9-[(1R,6R,8R,9S,10R,15S,17R,18S)-3,9,12,18-tetrakis(oxidanyl)-3,12-bis(oxidanylidene)-17-(6-oxidanylidene-3H-purin-9-yl)-2,4,7,11,13,16-hexaoxa-3$l^{5},12$l^{5}-diphosphatricyclo[13.3.0.0^{6,10}]octadecan-8-yl]-3H-purin-6-one | C20 H22 N8 O14 P2 | 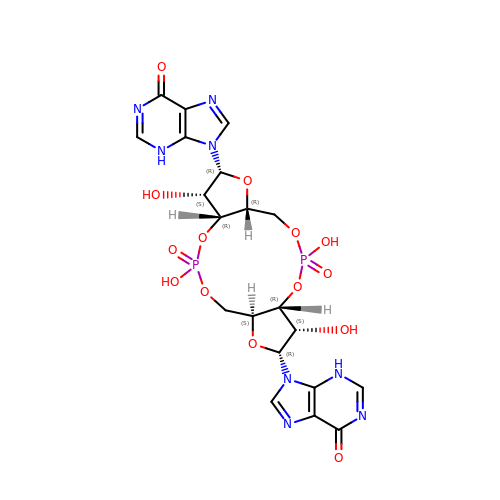VFTRASQVWRBMKD-PHSICLOESA-N>[2x]GAMGEPPLATRATAPPGVLKIFGAGLASGANYKSVLATARSTARELVAEALERYGLA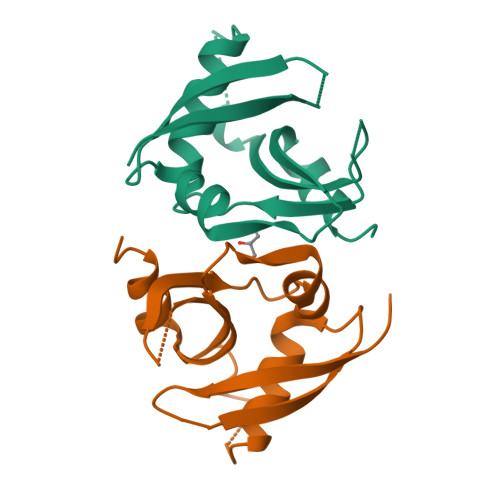GSPGGGPGESSCVDAFALCDALGRPAAAGVGSGEWRAEHLRVLGDSERPLLVQELWRARPGWARRFELRGREEARRLEQEAFGAADSEGTGAPSWRPQK> GPLSGLKKLIPEEGRELIGSVKKIIKRVSNEEKANEMEKNILKILIKVFFYIDSKAIQIGDLAKVDRALRDGFNHLDRAFRYYGVKKAADLVVILEKASTALKEAEQETVTLLTPFFRPHNIQLIRNTFAFLGSLDFFTKVWDDLEIEDDLFLLISALNKYTQIELIY

Therefore, Gip1 is a regulator of G protein shuttling between the membrane and the cytosol for wide-range chemotaxis. Gip1 consists of two regions, an N-terminal Pleckstrin-homology (PH) domain and a C-terminal region. The X-ray crystal structure of the C-terminal region of Gip1 shows cylinder-like folding with a central hydrophobic cavity. Mutagenesis and biochemical analyses indicate that the hydrophobic cavity and the hydrogen bond network at the entrance of the cavity are essential for complex formation with the geranylgeranyl modification on the Gγ subunit.

The two structures at 1.95 and 2.74 Å resolution were designated Form I and Form II. Gip1(146–310) consisted of seven α-helices designated α0 to α6 from the N terminus. Among them, helices α1 to α6 formed a cylinder-like structure with a centrally located hydrophobic cavity 22 Å in depth and 10 Å in diameter. We noticed that there was a tetrahedral area of electron density at the entrance of the cavity that extended to two long regions of electron. The lipid was surrounded by one water molecule and 22 residues that mostly formed hydrophobic interactions. In contrast to the hydrophobic interior, the surface of Gip1 was relatively charged without any notable hydrophobic regions. Second, our solved Gip1 structure contained bacterial glycerophospholipids, which suggests that the hydrophobic cavity is stably formed even without G proteins as cargo. Asp208 was one of the residues affected most severely by the substitutions and formed hydrogen bonds with both the side chain of Arg212 and the main chain nitrogen of Leu308 at the rim of the cavity entrance, which connected the C-terminal tail with the α3 helix. For example, the hydrogen bonding partners of aspartic acid, the 208th amino acid residue (Asp208), and Arg212 were Leu308 and Thr304 in Form I but Tyr303 in Form II. The hydrogen bond pattern changes are associated with different configurations of the C terminus of the α6 helix, including a directional change of the side chain at Glu307 (discussed later). This structural difference resulted in a slight change in the cavity shape and entrance.>MGSSHHHHHHSSENLYFQGHSLPGANSLTIRKDSNKYVTAHFMVGIVENYTVDDWKHDMELAKETGIDAFALNCASIDSYTDKQLAYAYEAAEEVDFKVFISFDFAYWSNGDTARITSIMQTYADHPGQFQYNGAALVSTFVGDSFDWGPVKRAVDHPIFAVPNLQDPNWAGHATTSIDGAFSWYAWPTDGGNSIIKGPMTTIWDDRFRNNLKDKVYMAPVSPWFSTHFNTKNWVFICEDLPHLRWQQMLEMQPELIEIISWNDYGESHYIGPYSEAHSDDGSAQWTKDFPHDAWRIIAKPYIAAYKAGEREPTVESDQLVYWYRPTPKAVTCSKDPLGPPNGINLLEDSVFVTTLLTEPATLTVGSGSLEFSVDVDAGIVTNSFPMGVGSQAFSVTRDGEEILGGDGGLDVQDRCDYYNFNVYVGSFSA[2x]

Glycoside hydrolase family 71 (GH71) includes α-1,3-glucan degrading enzymes which could be exploited for biotechnological applications; however, the family is presently poorly understood. To increase our understanding of GH71, we have performed a phylogenetic analysis of the family and detailed biochemical analysis of two of the five GH71 enzymes encoded by Aspergillus nidulans (AnGH71B and -C). We present the first structure of a GH71 protein, AnGH71C, including structures with carbohydrate ligands. These structures revealed a conserved acidic dyad (DxxE), found to be crucial for activity, and active site water coordination consistent with a classical inverting GH mechanism.

As no protein structural information is hitherto present for GH71 and to establish a greater fundamental understanding of the family, we pursued the structural determination of AnGH71C by macromolecular crystallography. The structure was solved to 1.33 Å resolution by molecular replacement using a model of the protein generated by AlphaFold232,33 and all residues of the protein could be modelled into the electron density map, except for 9 and 12 N-terminal residues in chains A and B, respectively, and the N-terminal His6 purification tag. Crystals of the apo protein and glucose-soaked crystals were of the C121 space group with similar unit cell dimensions and contained 2 molecules in the asymmetric unit, while the nigerotetraose soak was determined in P1 containing 4 molecules in the asymmetric unit. The protein contains an N-terminal (β/α)8 barrel, a short linker (9 residues), and a C-terminal β-sandwich comprised of 8 strands which packs along the side of the barrel. The β-sandwich domain has an immunoglobulin-like fold with a topology most closely related to Fibronectin type III (FnIII) members but contains an additional C-terminal β-strand (βE) compared to canonical members. The βE strand interacts with βA forming a four stranded sheet packing into a 4 × 4 sandwich which, to the best of our knowledge, is the first observation of such a topology. The interface in AnGH71C buries 21% of the sandwiches’ solvent accessible surface, as determined by analysis with PISA40, which includes several hydrophobic and aromatic residues along both faces and is stabilized by 14 hydrogen bonds and a salt bridge. The N-terminal (β/α)8-barrel domain is most closely related to GH99 (Cα RMSD between 2.8 and 3.1 to GH99 members), a family mainly containing retaining endo-α-1,2-mannanases as characterized members. The most distinct difference between the GH99 and GH71 (β/α)8-barrels is that AnGH71C lacks a region of ~50 residues found between β1 and α1 in the GH99 members, which forms a large loop wrapping one side of the substrate binding cleft.Nuclear pore complexes (NPCs) create large conduits for cargo transport between the nucleus and cytoplasm across the nuclear envelope (NE). These multi-megadalton structures are composed of about thirty different nucleoporins that are distributed in three main substructures (the inner, cytoplasmic and nucleoplasmic rings) around the central transport channel. Here we use cryo-electron tomography on DLD-1 cells that were prepared using cryo-focused-ion-beam milling to generate a structural model for the human NPC in its native environment. Our findings highlight the inherent flexibility of the NPC and suggest that the cellular environment has a considerable influence on NPC dimensions and architecture.

The nucleoplasmic ring (NR) shares scaffold nucleoporins (Nups) with the CR and anchors a distinct basket-like structure with diverse functions. For the NR and CR, we used a composite Y-complex model derived from overlapping crystal structures and threaded models. Bending at recognized ‘hinge points’, we fit the Y complex. It docks into both the CR and NR in a reticulated pattern of eight-membered rings. The principal Y-complex arrangement in both the CR and NR follows a reticulated pattern composed of two eight-membered rings. The NR is also composed of two eight-membered rings of Y complexes. In each ring, we observed considerable density beyond the Y complexes. In contrast to the IR, the diameters of the CR and NR are nearly identical to previous models. However, to accommodate a flatter overall assembly, the CR and NR rings flex in relation to the NE. At both the CR and NR, the Y-complex rings are angled more inward towards the central channel.

>[4x]MFPAAPSPRTPGTGSRRGPLAGLGPGSTPRTASRKGLPLGSAVSSPVLFSPVGRRSSLSSRGTPTRMFPHHSITESVNYDVKTFGSSLPVKVMEALTLAEVDDQLTINIDEGGWACLVCKEKLIIWKIALSPITKLSVCKELQLPPSDFHWSADLVALSYSSPSGEAHSTQAVAVMVATREGSIRYWPSLAGEDTYTEAFVDSGGDKTYSFLTAVQGGSFILSSSGSQLIRLIPESSGKIHQHILPQGQGMLSGIGRKVSSLFGILSPSSDLTLSSVLWDRERSSFYSLTSSNISKWELDDSSEKHAYSWDINRALKENITDAIWGSESNYEAIKEGVNIRYLDLKQNCDGLVILAAAWHSADNPCLIYYSLITIEDNGCQMSDAVTVEVTQYNPPFQSEDLILCQLTVPNFSNQTAYLYNESAVYVCSTGTGKFSLPQEKIVFNAQGDSVLGAGACGGVPIIFSRNSGLVSITSRENVSILAEDLEGSLASSVAGPNSESMIFETTTKNETIAQEDKIKLLKAAFLQYCRKDLGHAQMVVDELFSSHSDLDSDSELDRAVTQISVDLMDDYPASDPRWAESVPEEAPGFSNTSLIILHQLEDKMKAHSFLMDFIHQVGLFGRLGSFPVRGTPMATRLLLCEHAEKLSAAIVLKNHHSRLSDLVNTAILIALNKREYEIPSNLTPADVFFREVSQVDTICECLLEHEEQVLRDAPMDSIEWAEVVINVNNILKDMLQAASHYRQNRNSLYRREESLEKEPEYVPWTATSGPGGIRTVIIRQHEIVLKVAYPQADSNLRNIVTEQLVALIDCFLDGYVSQLKSVDKSSNRERYDNLEMEYLQKRSDLLSPLLSLGQYLWAASLAEKYCDFDILVQMCEQTDNQSRLQRYMTQFADQNFSDFLFRWYLEKGKRGKLLSQPISQHGQLANFLQAHEHLSWLHEINSQELEKAHATLLGLANMETRYFAKKKTLLGLSKLAALASDFSEDMLQEKIEEMAEQERFLLHQETLPEQLLAEKQLNLSAMPVLTAPQLIGLYICEENRRANEYDFKKALDLLEYIDEEEDININDLKLEILCKALQRDNWSSSDGKDDPIEVSKDSIFVKILQKLLKDGIQLSEYLPEVKDLLQADQLGSLKSNPYFEFVLKANYEYYVQGQI;>[4x]MDRSGFGEISSPVIREAEVTRTARKQSAQKRVLLQASQDENFGNTTPRNQVIPRTPSSFRQPFTPTSRSLLRQPDISCILGTGGKSPRLTQSSGFFGNLSMVTNLDDSNWAAAFSSQRSGLFTNTEPHSITEDVTISAVMLREDDPGEAASMSMFSDFLQSFLKHSSSTVFDLVEEYENICGSQVNILSKIVSRATPGLQKFSKTASMLWLLQQEMVTWRLLASLYRDRIQSALEEESVFAVTAVNASEKTVVEALFQRDSLVRQSQLVVDWLESIAKDEIGEFSDNIEFYAKSVYWENTLHTLKQRQLTSYVGSVRPLVTELDPDAPIRQKMPLDDLDREDEVRLLKYLFTLIRAGMTEEAQRLCKRCGQAWRAATLEGWKLYHDPNVNGGTELEPVEGNPYRRIWKISCWRMAEDELFNRYERAIYAALSGNLKQLLPVCDTWEDTVWAYFRVMVDSLVEQEIQTSVATLDETEELPREYLGANWTLEKVFEELQATDKKRVLEENQEHYHIVQKFLILGDIDGLMDEFSKWLSKSRNNLPGHLLRFMTHLILFFRTLGLQTKEEVSIEVLKTYIQLLIREKHTNLIAFYTCHLPQDLAVAQYALFLESVTEFEQRHHCLELAKEADLDVATITKTVVENIRKKDNGEFSHHDLAPALDTGTTEEDRLKIDVIDWLVFDPAQRAEALKQGNAIMRKFLASKKHEAAKEVFVKIPQDSIAEIYNQCEEQGMESPLPAEDDNAIREHLCIRAYLEAHETFNEWFKHMNSVPQKPALIPQPTFTEKVAHEHKEKKYEMDFGIWKGHLDALTADVKEKMYNVLLFVDGGWMVDVREDAKEDHERTHQMVLLRKLCLPMLCFLLHTILHSTGQYQECLQLADMVSSERHKLYLVFSKEELRKLLQKLRESSLMLLDQGLDPLGYEIQL;>SKYGLQDSDEEEEEHPSKTSTKKLKTAPLPPASQTTPLQMALNGKPAPPPQSQSPEVEQLGRVVELDSDMVDITQEPVLDTMLEESMPEDQEPVSASTHIASSLGINPHVLQIMKASLLTDEEDVDMALDQRFSRLPSKADTSQEICSPRLPISASHSSKTRSLVGGLLQSKFTSGAFLSPSVSVQECRTPRAASLMNIPSTSSWSVPPPLTSVFTMPSPAPEVPLKTVGTRRQLGLVPREKSVTYGKGKLLMDMALFMGRSFRVGWGPNWTLANSGEQLNGSHELENHQIADSMEFGFLPNPVAVKPLTESPFKVHLEKLSLRQRKPDEDMKLYQTPLELKLKHSTVHVDELCPLIVPNLGVAVIHDYADWVKEASGDLPEAQIVKHWSLTWTLCEALWGHLKELDSQLNEPREYIQILERRRAFSRWLSCTATPQIEEEVSLTQKNSPVEAVFSYLTGKRISEACSLAQQSGDHRLALLLSQFVGSQSVRELLTMQLVDWHQLQADSFIQDERLRIFALLAGKPVWQLSEKKQINVCSQLDWKRSLAIHLWYLLPPTASISRALSMYEEAFQNTSDSDRYACSPLPSYLEGSGCVIAEEQNSQTPLRDVCFHLLKLYSDRHYDLNQLLEPRSITADPLDYRLSWHLWEVLRALNYTHLSAQCEGVLQASYAGQLESEGLWEWAIFVLLHIDNSGIREKAVRELLTRHCQLLETPESWAKETFLTQKLRVPAKWIHEAKAVRAHMESDKHLEALCLFKAEHWNRCHKLIIRHLASDAIINENYDYLKGFLEDLAPPERSSLIQDWETSGLVYLDYIRVIEMLRHIQQVDCSGNDLEQLHIKVTSLCSRIEQIQCYSAKDRLAQSDMAKRVANLLRVVLSLHHPPDRTSDSTPDPQRVPLRLLAPHIGRLPMPEDYAMDELRSLTQSYLRELAVGSL[4x];>[4x]MVSVINTVDTSHEDMIHDAQMDYYGTRLATCSSDRSVKIFDVRNGGQILIADLRGHEGPVWQVAWAHPMYGNILASCSYDRKVIIWREENGTWEKSHEHAGHDSSVNSVCWAPHDYGLILACGSSDGAISLLTYTGEGQWEVKKINNAHTIGCNAVSWAPAVVPGSLIDHPSGQKPNYIKRFASGGCDNLIKLWKEEEDGQWKEEQKLEAHSDWVRDVAWAPSIGLPTSTIASCSQDGRVFIWTCDDASSNTWSPKLLHKFNDVVWHVSWSITANILAVSGGDNKVTLWKESVDGQWVCISDVNKGQGSVSASVTEGQQNEQ;>MFVARSIAADHKDLIHDVSFDFHGRRMATCSSDQSVKVWDKSESGDWHCTASWKTHSGSVWRVTWAHPEFGQVLASCSFDRTAAVWEEIVGESNDKLRGQSHWVKRTTLVDSRTSVTDVKFAPKHMGLMLATCSADGIVRIYEAPDVMNLSQWSLQHEISCKLSCSCISWNPSSSRAHSPMIAVGSDDSSPNAMAKVQIFEYNENTRKYAKAETLMTVTDPVHDIAFAPNLGRSFHILAIATKDVRIFTLKPVRKELTSSGGPTKFEIHIVAQFDNHNSQVWRVSWNITGTVLASSGDDGCVRLWKANYMDNWKCTGILKGNGSPVNGSSQQGTSNPSLGSTIPSLQNSLNGSSAGRKHS[4x];>[4x]MEELDGEPTVTLIPGVNSKKNQMYFDWGPGEMLVCETSFNKKEKSEMVPSCPFIYIIRKDVDVYSQILRKLFNESHGIFLGLQRIDEELTGKSRKSQLVRVSKNYRSVIRACMEEMHQVAIAAKDPANGRQFSSQVSILSAMELIWNLCEILFIEVAPAGPLLLHLLDWVRLHVCEVDSLSADVLGSENPSKHDSFWNLVTILVLQGRLDEARQMLSKEADASPASAGICRIMGDLMRTMPILSPGNTQTLTELELKWQHWHEECERYLQDSTFATSPHLESLLKIMLGDEAALLEQKELLSNWYHFLVTRLLYSNPTVKPIDLHYYAQSSLDLFLGGESSPEPLDNILLAAFEFDIHQVIKECSIALSNWWFVAHLTDLLDHCKLLQSHNLYFGSNMREFLLLEYASGLFAHPSLWQLGVDYFDYCPELGRVSLELHIERIPLNTEQKALKVLRICEQRQMTEQVRSICKILAMKAVRNNRLGSALSWSIRAKDAAFATLVSDRFLRDYCERGCFSDLDLIDNLGPAMMLSDRLTFLGKYREFHRMYGEKRFADAASLLLSLMTSRIAPRSFWMTLLTDALPLLEQKQVIFSAEQTYELMRCLEDLTSRRPVHGESDTEQLQDDDIETTKVEMLRLSLARNLARAIIREGSLEGS;>[4x]MEEIYAKFVSQKISKTRWRPLPPGSLQTAETFATGSWDNEENYISLWSIGDFGNLDSDGGFEGDHQLLCDIRHHGDVMDLQFFDQERIVAASSTGCVTVFLHHPNNQTLSVNQQWTTAHYHTGPGSPSYSSAPCTGVVCNNPEIVTVGEDGRINLFRADHKEAVRTIDNADSSTLHAVTFLRTPEILTVNSIGQLKIWDFRQQGNEPSQILSLTGDRVPLHCVDRHPNQQHVVATGGQDGMLSIWDVRQGTMPVSLLKAHEAEMWEVHFHPSNPEHLFTCSEDGSLWHWDASTDVPEKSSLFHQGGRSSTFLSHSISNQANVHQSVISSWLSTDPAKDRIEITSLLPSRSLSVNTLDVLGPCLVCGTDAEAIYVTRHLFS;>MLHLSAAPPAPPPEVTATARPCLCSVGRRGDGGKMAAAGALERSFVELSGAERERPRHFREFTVCSIGTANAVAGAVKYSESAGGFYYVESGKLFSVTRNRFIHWKTSGDTLELMEESLDINLLNNAIRLKFQNCSVLPGGVYVSETQNRVIILMLTNQTVHRLLLPHPSRMYRSELVVDSQMQSIFTDIGKVDFTDPCNYQLIPAVPGISPNSTASTAWLSSDGEALFALPCASGGIFVLKLPPYDIPGMVSVVELKQSSVMQRLLTGWMPTAIRGDQSPSDRPLSLAVHCVEHDAFIFALCQDHKLRMWSYKEQMCLMVADMLEYVPVKKDLRLTAGTGHKLRLAYSPTMGLYLGIYMHAPKRGQFCIFQLVSTESNRYSLDHISSLFTSQETLIDFALTSTDIWALWHDAENQTVVKYINFEHNVAGQWNPVFMQPLPEEEIVIRDDQDPREMYLQSLFTPGQFTNEALCKALQIFCRGTERNLDLSWSELKKEVTLAVENELQGSVTEYEFSQEEFRNLQQEFWCKFYACCLQYQEALSHPLALHLNPHTNMVCLLKKGYLSFLIPSSLVDHLYLLPYENLLTEDETTISDDVDIARDVICLIKCLRLIEESVTVDMSVIMEMSCYNLQSPEKAAEQILEDMITIDVENVMEDICSKLQEIRNPIHAIGLLIREMDYETEVEMEKGFNPAQPLNIRMNLTQLYGSNTAGYIVCRGVHKIASTRFLICRDLLILQQLLMRLGDAVIWGTGQLFQAQQDLLHRTAPLLLSYYLIKWGSECLATDVPLDTLESNLQHLSVLELTDSGALMANRFVSSPQTIVELFFQEVARKHIISHLFSQPKAPLSQTGLNWPEMITAITSYLLQLLWPSNPGCLFLECLMGNCQYVQLQDYIQLLHPWCQVNVGSCRFMLGRCYLVTGEGQKALECFCQAASEVGKEEFLDRLIRSEDGEIVSTPRLQYYDKVLRLLDVIGLPELVIQLATSAITEAGDDWKSQATLRTCIFKHHLDLGHNSQAYEALTQIPDSSRQLDCLRQLVVVLCERSQLQDLVEFPYVNLHNEVVGIIESRARAVDLMTHNYYELLYAFHIYRHNYRKAGTVMFEYGMRLGREVRTLRGLEKQGNCYLAALNCLRLIRPEYAWIVQPVSGAVYDRPGASPKRNHDGECTAAPTNRQIEILELEDLEKECSLARIRLTLAQHDPSAVAVAGSSSAEEMVTLLVQAGLFDTAISLCQTFKLPLTPVFEGLAFKCIKLQFGGEAAQAEAWAWLAANQLSSVITTKESSATDEAWRLLSTYLERYKVQNNLYHHCVINKLLSHGVPLPNWLINSYKKVDAAELLRLYLNYDLLEEAVDLVSEYVDAVLGKGHQYFGIEFPLSATAPMVWLPYSSIDQLLQALGENSANSHNIALSQKILDKLEDYQQKVDKATRDLLYRRTL[4x];>MKQDASRNAAYTVDCEDYVHVVEFNPFENGDSGNLIAYGGNNYVVIGTCTFQEEEADVEGIQYKTLRTFHHGVRVDGIAWSPETRLDSLPPVIKFCTSAADMKIRLFTSDLQDKNEYKVLEGHTDFINGLVFDPKEGQEIASVSDDHTCRIWNLEGVQTAHFVLHSPGMSVCWHPEETFKLMVAEKNGTIRFYDLLAQQAILSLESEQVPLMSAHWCLKNTFKVGAVAGNDWLIWDITRSSYPQNKRPVHMDRACLFRWSTISENLFATTGYPGKMASQFQIHHLGHPQPILMGSVAVGSGLSWHRTLPLCVIGGDHKLLFWVTEV[4x]5-(DIMETHYLAMINO)-1-NAPHTHALENESULFONIC 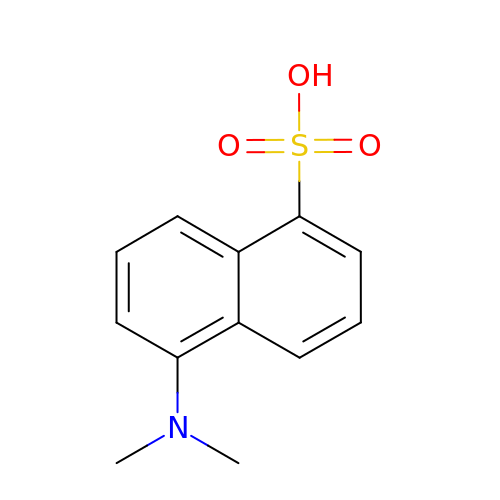ACID(DANSYL ACID) | C12 H13 N O3 S | BBEQQKBWUHCIOU-UHFFFAOYSA-N(4aR,8aS)-8a-(2,4-difluorophenyl)-4,4a,5,6,8,8a-hexahydropyrano[3,4-d][1,3]thiazin-2-amine 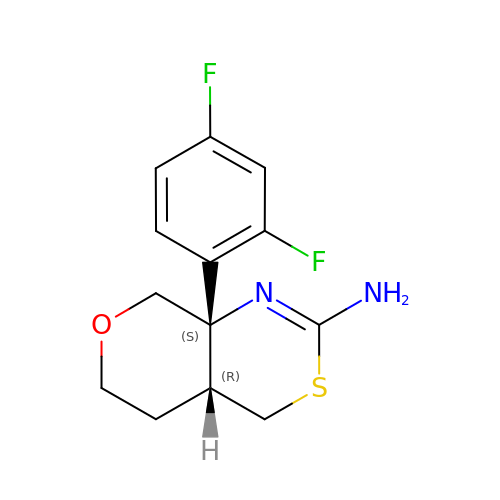| C13 H14 F2 N2 O S | CUNQNADGWRXYCV-SDBXPKJASA-N>[2x]FVLKTPKGTRDYSPRQMAVREKVFDVIIRCFKRHGAEVIDTPVFELKETLMGKYGEDSKLIYDLKDQGGELLSLRYDLTVPFARYLAMNKLTNIKRYHIAKVYRRDNPAMTRGRYREFYQCEFDIAGNFDPMIPDAECLKIMCEILSSLQIGDFLVKVNDRRILDGMFAICGVSDSKFRTICSSVDKLDKVSWEEVKNEMVGEKGLAPEVADRIGDYVQQHGGVSLVEQLLQDPKLSQN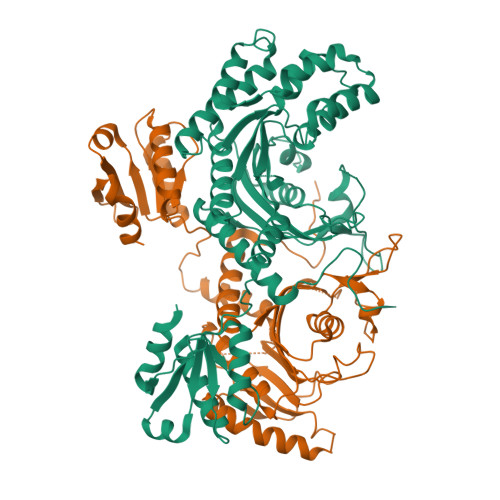KQALEGLGDLKLLFEYLTLFGIDDKISFDLSLARGLDYYTGVIYEAVLLQTPAQAGEEPLGVGSVAAGGRYDGLVGMFDPKGRKVPCVGLSIGVERIFSIVEQRLEALEEKIRTTETQVLVASAQKKLLEERLKLVSELWDAGIKAELLYKKNPKLLNQLQYCEEAGIPLVAIIGEQELKDGVIKLRSVTSREEVDVRREDLVEEIKRRTG>SLRSDLINALYDENQKYDVCGIISAEGKIYPLGSDTKVLSTIFELFSRPIINKIAEKHGYIVEEPKQQNHYPDFTLYKPSEPNKKIAIDIKTTYTNKENEKIKFTLGGYTSFIRNNTKNIVYPFDQYIAHWIIGYVYTRVATRKSSLKTYNINELNEIPKPYKGVKV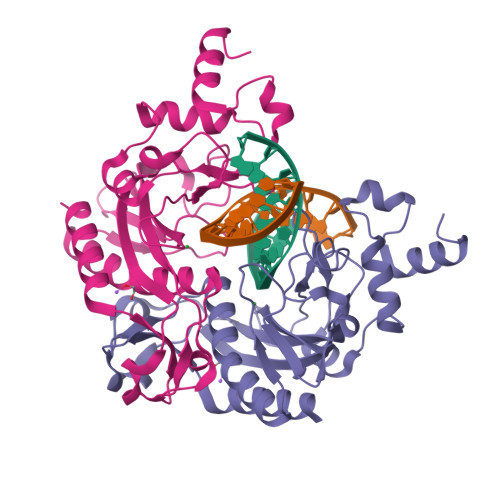FLQDKWVIAGDLAGSGNTTNIGSIHAHYKDFVEGKGIFDSEDEFLDYWRNYERTSQLRNDKYNNISEYRNWIYRGRK[2x]>MGSSHHHHHHSGLVPRGSHMAGARTQELVQQRTQGLLEKVINERLVALARAQVSQIQRELEYPLTVVHGLANSTRLLGEPGADGMPQLNASRDEISALLRSTVQNNPKLLDTFMAWEPNAFDTDAAFAGQPGKGYGPDGRYLPWWYRGADGKPIVEAMADSIDSEKLLPTGVRENEFYACPKENKRPCIIDPAPYEMGGKTVMMSSFNVPIMVGDQFRGAVGADLSLAFIQDLLKRADQQLYDGAGEMALIASNGRLVAYTRDDSKLGEPAGSVLD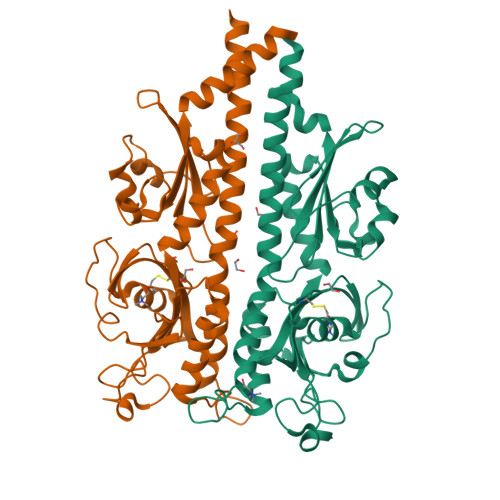GNEVDNLKNLTVDQPLYDIDAEHGHIELFLPFTIADSGVRWTLMLQIPQAAVFGELQQLQGELSDQRQQDILGM[2x]(2~{S})-2-azanyl-3-(9-oxidanylidene-10~{H}-acridin-2-yl)propanoic 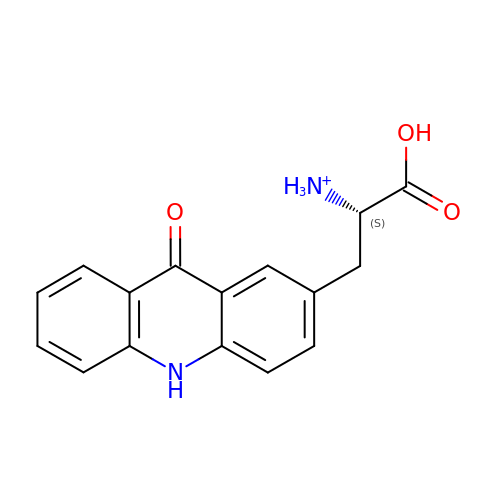acid | C16 H15 N2 O3 | NPALYBYZIAGBTE-LBPRGKRZSA-O> MSTDVAAAQAQSKIDLTKKK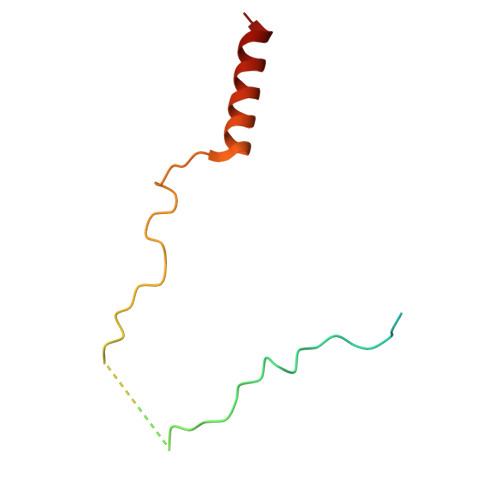NEEINKKSLEEDDEFEDFPIDTWANGETIKSNAVTQTNIWEENWDDVEVDDDFTNELKAELDRYKRENQ> GPGSH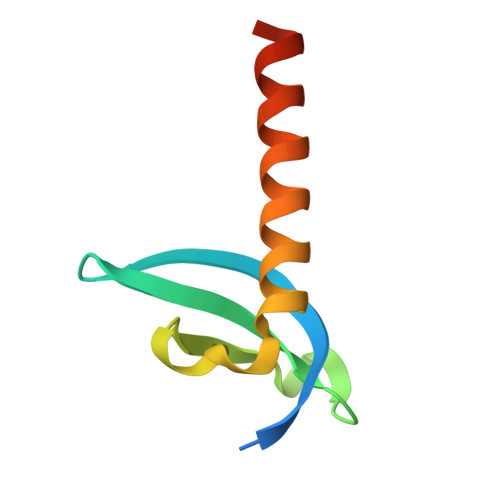VEEYVVEKILGKRFVNGRPQVLVKWSGFPNENNTWEPLENVGNCMKLVSDFESEVFRLHRKAAAKSVGKS2,6-anhydro-1,4-dideoxy-1-[4-(4-fluorophenyl)-1H-1,2,3-triazol-1-yl]-4-(4-phenyl-1H-1,2,3-triazol-1-yl)-D-glycero-L-manno-heptitol 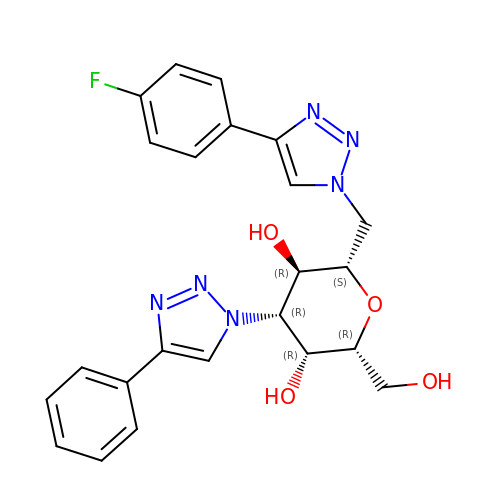| C23 H23 F N6 O4 | SRBNPRKOXDJHBB-NQQQLTFYSA-N>GSHMSGTEEAILGGRDSHPAAGGGSVLCFGQCQYTAEEYQAIQKALRQRLGPEYISSRMAGGGQKVCYIEGHRVINLANEMFGYNGWAHSITQQNVDFVDLNNGAFYVGVCAFVRVQLKDGSYHEDVGYGVSEGLASKALSLEKARKEAVTDGLKRALRSFGNALGNCILDKDYLRSLNKLPRQLPLEVDLTKAK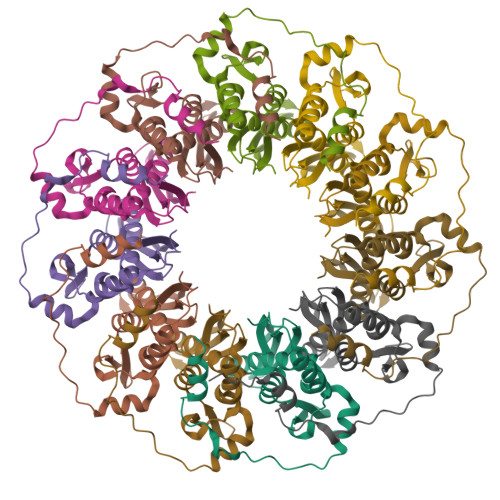RQDLEPSVEAARYNSCRPNM[11x]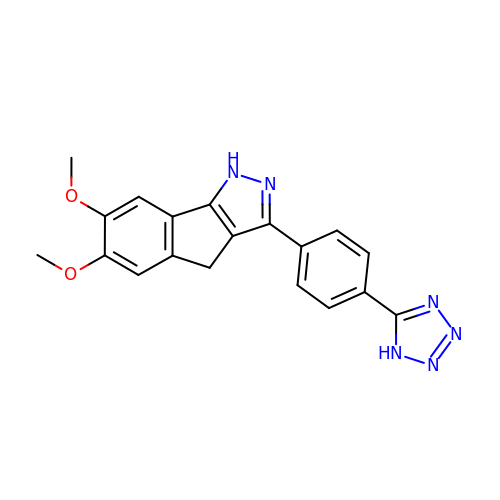6,7-dimethoxy-3-[4-(1H-tetrazol-5-yl)phenyl]-1,4-dihydroindeno[1,2-c]pyrazole | C19 H16 N6 O2 | NDAAHSGATZAMOW-UHFFFAOYSA-N>[2x]PVNPCCYYPCQHQGICVRFGLDRYQCDCTRTGYSGPNCTIPEIWTWLRTTLRPSPSFIHFLLTHGRWLWDFVNATFIRDTLMRLVLTVRSNLIPSPPTYNIAHDYISWESFSNVSYYTRI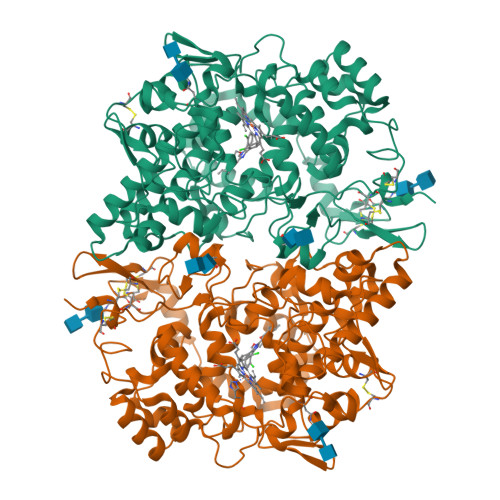LPSVPRDCPTPMDTKGKKQLPDAEFLSRRFLLRRKFIPDPQSTNLMFAFFAQHFTHQFFKTSGKMGPGFTKALGHGVDLGHIYGDNLERQYQLRLFKDGKLKYQMLNGEVYPPSVEEAPVLMHYPRGIPPQSQMAVGQEVFGLLPGLMLYATIWLREHNRVCDLLKAEHPTWGDEQLFQTARLILIGETIKIVIEEYVQQLSGYFLQLKFDPELLFGAQFQYRNRIAMEFNQLYHWHPLMPDSFRVGPQDYSYEQFLFNTSMLVDYGVEALVDAFSRQPAGRIGGGRNIDHHILHVAVDVIKESRVLRLQPFNEYRKRFGMKPYTSFQELTGEKEMAAELEELYGDIDALEFYPGLLLEKCHPNSIFGESMIEMGAPFSLKGLLGNPICSPEYWKASTFGGEVGFNLVKTATLKKLVCLNTKTCPYVSFHVPD>ARKCSLTGKWTNDLGSNMTIGAVNSRGEFTGTYTTAVTATSNEIKES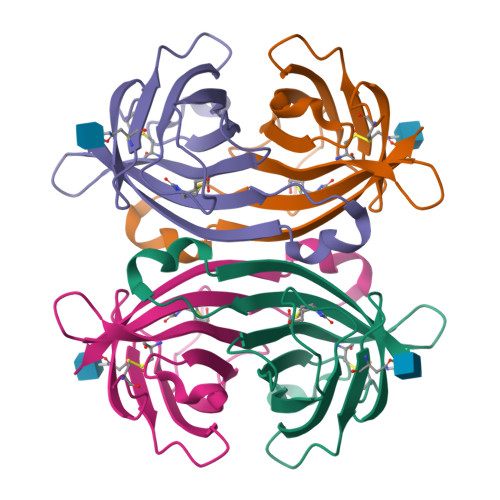PLHGTENTINKRTQPTFGFTVNWKFSESTTVFTGQCFIDRNGKEVLKTMWLLRSSVNDIGDDWKATRVGINIFTRLRTQKE[2x]>[8x]MPSPPGNLRVTDVTSTSVTL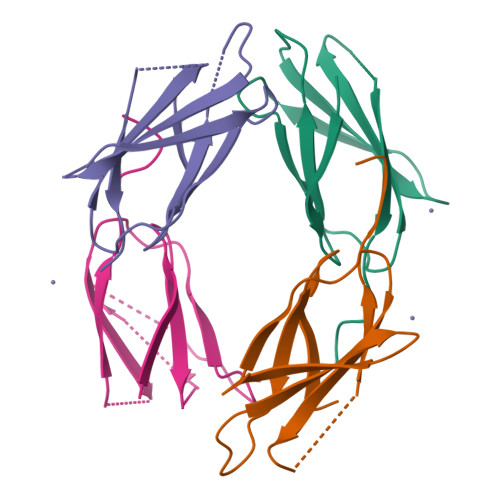SWRGYPWATGYRVEYREAGGEWKEVTVPGDLSHRYTVTGLKPGTEYEFRVRAVNRVGRTFDTPGPSSVSVTTGHHHHHH> GAMDYKDDDDKKTNWLKRIYRVRPCVKCKVAPRNWKVKNKHLRIYNMCKTCFNNSIDIGDDT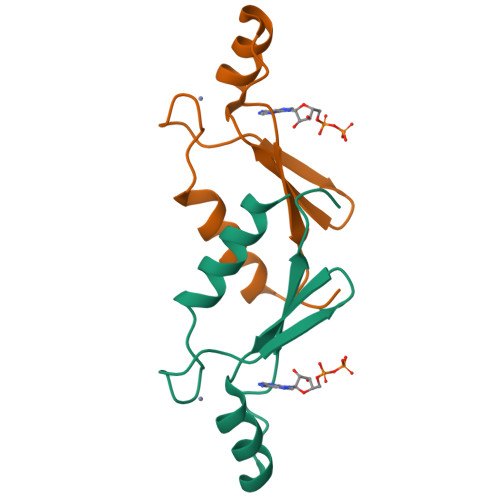YHGHDDWLMYADSKEISN> MGSSHHHHHHSSGLVPRGSHMTTTISADQVNQIIYNLHHDPFEILGCHLLEEGKNTKKWVVRAYLPKAEAAWVIRPTERKEDPMNSVHHPNFFECIIETPELNHYQLKVKEGEHEKVIYDPYAFSSPYLTDEDIYLFSEGNHHRIYEKLGAHVGEINGVKGVYFAVWAPNARNVSVIGDFNNWDGREHQMRKRNYTIWELFVPEIGSGTVYKYEIKNSEGHIYEKSDPYGFYREVRPNTASIVVDIDNIYQWHDEEWLEKRRNSDPLKQPVSVYEVHLGSWLHGSSAEKMPLLNGEADPVIVSEWNPGARFLSYYELAEKLIPYVKDMGYTHIELLPIAEHPFDGSWGYQVTGFYSPTSRFGRPEDFMYFVDKCHENGIGVILDWVPGHFPKDSHGLAYFDGTHLYEHADPRIGEHKEWGTLVFNYGRHEVRNFLVANVLFWFDKYHVDGIRVDAVASMLYRNYLRKEGEWIANEYGGDEHIEAVSFIREVNTLLFEYFPGILSIAEESTEWEKVSRPVYDGGLGFNLKWDMGWMHDMLDYFNIDPYFRQYHQNNVTFSMLYYYNENFMLALSHDEIVHGKSNMLGKMP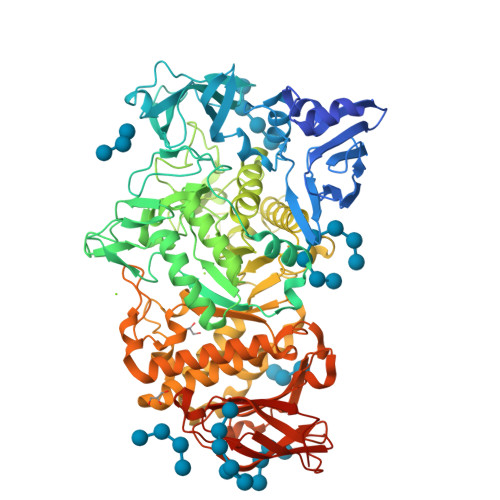GDEWQKYANVRALFTYMYTHPGKKTMFMSMEFGQWSEWNVWGDLEWHLLQYEPHQQLKQFFTDLNALYQQEPALYTHDFEYHGFEWIDCNDNTHSVVSFLRRSDDPNDSLVVVCNFTPQPHSHYRIGVPEAGYYVELFNSDAKQYGGSNMGNLGGKWADEWSFHNKPYSLDLCLPPLAVLILKLDPTKVPEGTTIKEIAADEEE>[2x]MLVVPAIDLFRGKVARMIKGRKENTIFYEKDPVELVEKLIEEGFTLIHVVDLSNAIENSGENLPVLEKLSEFAEH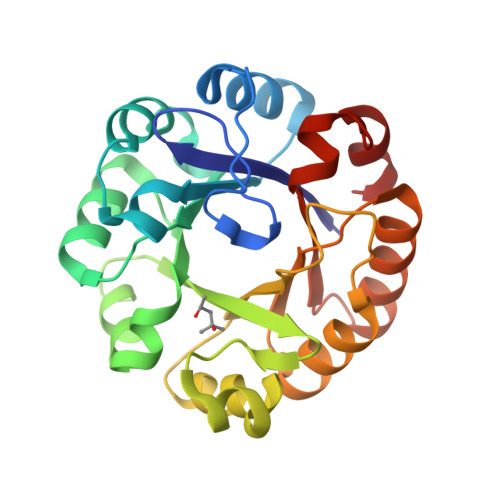IQIGGGIRSLDYAEKLRKLGYRRQIVSSKVLEDPSFLKSLREIDVEPVFSLVTRGGRVAFKGWLAEEEIDPVSLLKRLKEYGLEEIVHTEIEKDGTLQEHDFSLTKKIAIEAEVKVLAAGGISSENSLKTAQKVHTETNGLLKGVIVGRAFLEGILTVEVMKRYAR> VVVEIGKVTGSVGTTVEIPVYFRGVPSKGIANCDFVFRYDPNVLEIIGIDPGDIIVDPNPTKSFDTAIYPDRKIIVFLFAEDSGTGAYAITKD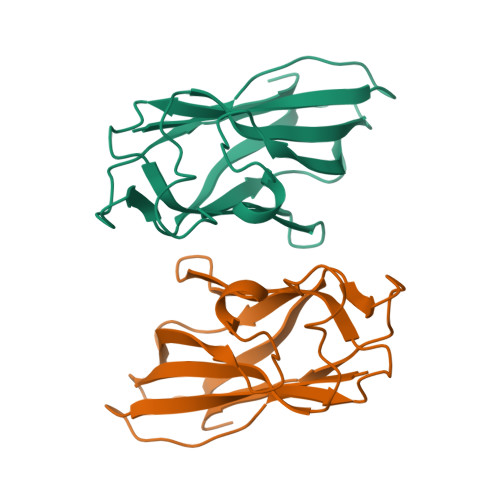GVFAKIRATVKSSAPGYITFDEVGGFADNDLVEQKVSFIDGGVNV>XASCSXGPN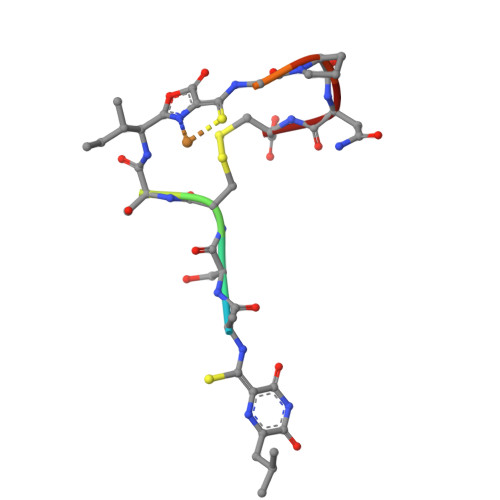C[2x]>[3x]AAKELTLAQTESLRE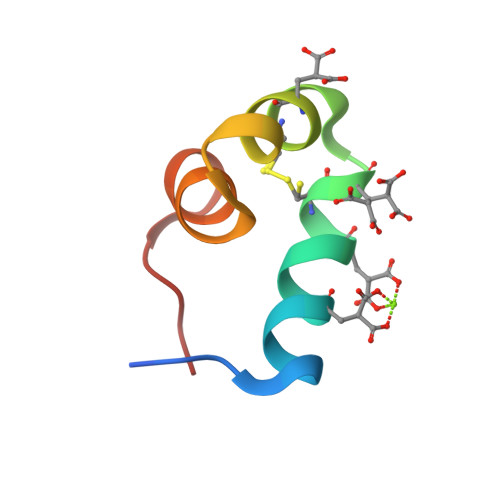VCETNMACDEMADAQGIVAAYQAFYGPIPF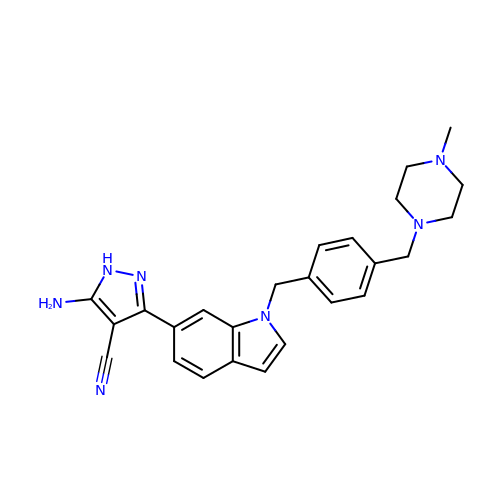5-azanyl-3-[1-[[4-[(4-methylpiperazin-1-yl)methyl]phenyl]methyl]indol-6-yl]-1~{H}-pyrazole-4-carbonitrile | C25 H27 N7 | DTFOFBCTICVEIL-UHFFFAOYSA-N> MTAPASHYTFANLKKLGLCAPQVALSRQPRLRPHVGHLNGLVYPLPYYAMWRGNHDKYTYNQATPARW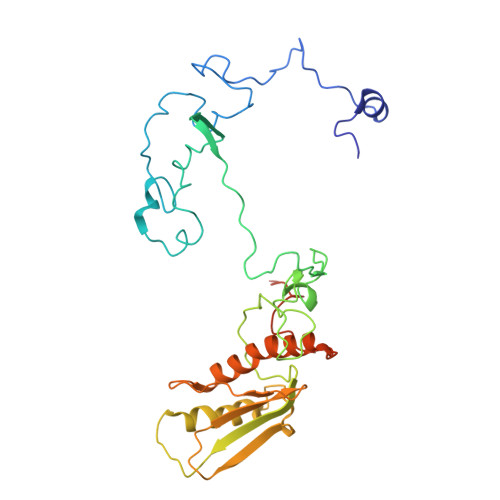GEGNTNTMYHQHYAHAKCPTDYGRGGREFQFLSVKRGKLKRKPLPTVQYVDPNSKPQWVFKSWHNPLSAPSMWEREVQYPEHTPAHTGAKRPLAVVAPKTSHKHLFLMHMEKVTVTVSPLLFGYGHTLQKAALDFYRRGLSARSPFPSDKMFLYYSIDHITPKIEVTWLDGSVYVPPLIEGVKAQDLIQMVMEQAWLAADRMSAEGRVLNPIAIDDYKWEQLIAFKQKRAKGAEAAKGGAKKK>MIIVYTTFPDWESAEKVVKTLLKERLIACANLREHRAFYWWEGKIEEDKEVGAILKTREALWEELKERIKEL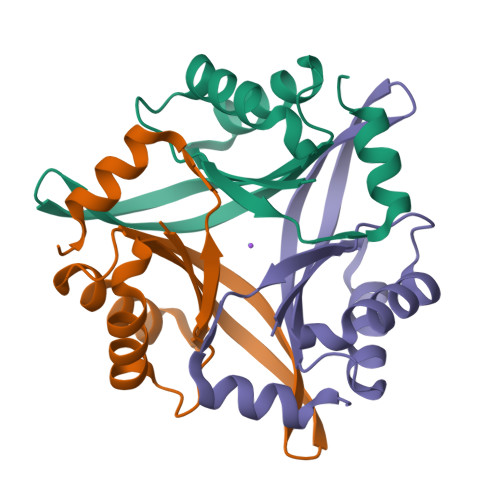HPYDVPAIIRIDVDDVNEDYLKWLIEETKK[3x]> MAIDLFCYLSIDRGAAESDLNKIRSNHSELFEGKFLISPVRDADFSLKEIAAEHGLVAE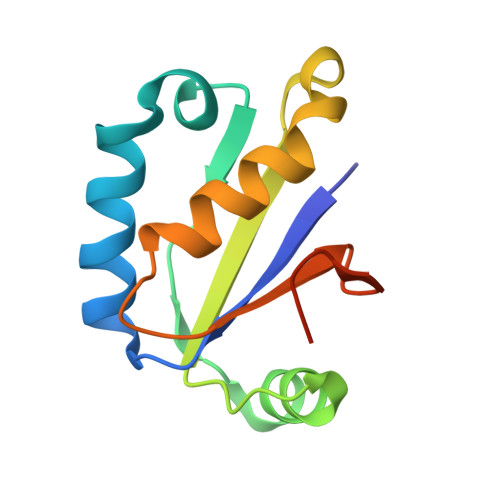SFFLVSLNDKNSADLIPIVSKILVDGFNGGAILILQDNEYRRTSLEHHHHHH(~{Z})-3-(1-benzothiophen-3-yl)-2-sulfanyl-prop-2-enoic acid | C11 H8 O2 S2 | 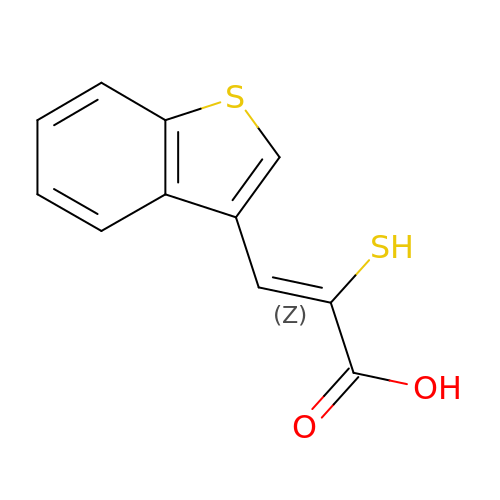RAMCKYVBVNEIFT-UITAMQMPSA-N> GYSLFPNSPKWTSKVVTYRIVSYTRDLPHITVDRLVSKALNMWGKEIPLHFRKVVWGTADIMIGFARGAHGDSYPFDGPGNTLAHAFAPGTGLGGDAHFDEDERWTDGSSLGI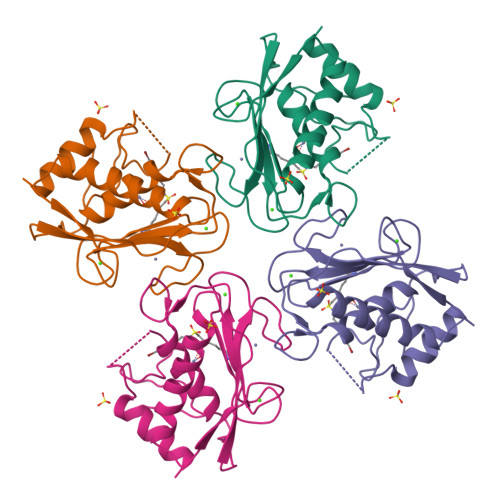NFLYAATHELGHSLGMGHSSDPNAVMYPTYGNGDPQNFKLSQDDIKGIQKLYGKRSNSRKK N-acetyl-S-[(1S)-1,2-dichloroethyl]-L-cysteine | C7 H11 Cl2 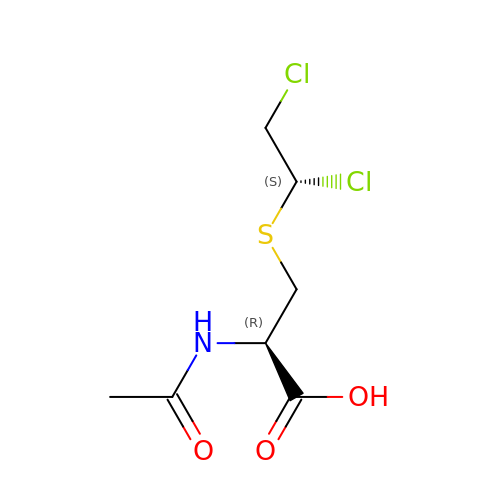N O3 S | IORNBBWVBAMRIG-NTSWFWBYSA-N> MEDENILRNAVNLQVLKFHYPEIESIIDIASHVAVYQFDVGSQKWLKTSIEGTFFLVKDQRARVGY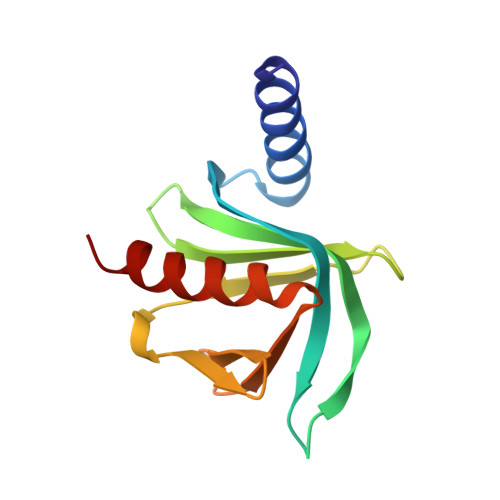VILNRNSPENLYLFINHPSNVHLVDRYLIHRTENQHVVGLWMFDPNDMSRIFNIVKESLLR>[4x]MKQIKKLLVANRGEIAIRIFRAAAELDISTVAIYSNEDKSSLHRYKADESYLVGSDLGPAESYLNIERIIDVAKQANVDAIHPGYGFLSENEQFARRCAEEGIKFIGPHLEHLDMFGDKVKARTTAIKADLPVIPGTDGPIKSYELAKEFAEEAGFPLMIKATSGGGGKGMRIVREESELEDAFHRAKSEAEKSFGNSEVYIERYIDNPKHIEVQVIGDEHGNIVHLFERDCSVQRRHQKVVEVAPSVGLSPTLRQRICDAAIQLMENIKYVNAGTVEFLVSGDEFFFIEVNPRVQVEHTITEMVTGIDIVKTQILVAAGADLFGEEINMPQQKDITTLGYAIQCRITTEDPLNDFMPDTGTIIAYRSSGGFGVRLDAGDGFQGAEISPYYDSLLVKLSTHAISFKQAEEKMVRSLREMRIRGVKTNIPFLINVMKNKKFTSGDYTTKFIEETPELFDIQPSLDRGTKTLEYIGNVTINGFPNVEKRPKPDYELASIPTVSSSKIASFSGTKQLLDEVGPKGVAEWVKKQDDVLLTDTTFRDAHQSLLATRVRTKDMINIASKTADVFKDGFSLEMWGGATFDVAYNFLKENPWERLERLRKAIPNVLFQMLLRASNAVGYKNYPDNVIHKFVQESAKAGIDVFRIFDSLNWVDQMKVANEAVQEAGKISEGTICYTGDILNPERSNIYTLEYYVKLAKELEREGFHILAIKDMAGLLKPKAAYELIGELKSAVDLPIHLHTHDTSGNGLLTYKQAIDAGVDIIDTAVASMSGLTSQPSANSLYYALNGFPRHLRTDIEGMESLSHYWSTVRTYYSDFESDIKSPNTEIYQHEMPGGQYSNLSQQAKSLGLGERFDEVKDMYRRVNFLFGDIVKVAPSSKVVGDMALYMVQNDLDEQSVITDGYKLDFPESVVSFFKGEIGQPVNGFNKDLQAVILK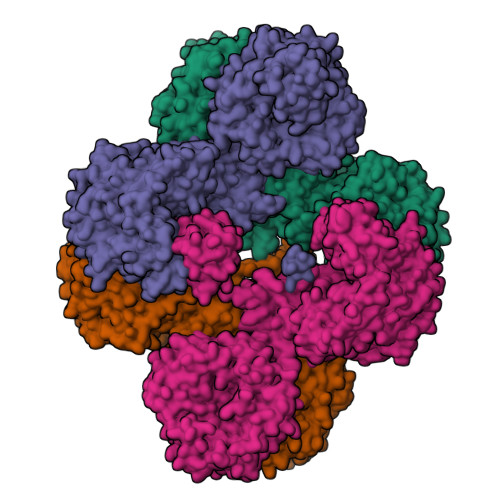GQEALTARPGEYLEPVDFEKVRELLEEEQQGPVTEQDIISYVLYPKVYEQYIQTRNQYGNLSLLDTPTFFFGMRNGETVEIEIDKGKRLIIKLETISEPDENGNRTIYYAMNGQARRIYIKDENVHTNANVKPKADKSNPSHIGAQMPGSVTEVKVSVGETVKANQPLLITEAMKMETTIQAPFDGVIKQVTVNNGDTIATGDLLIEIEKATD>[2x]MIKVEIKPSQAQFTTRSGVSR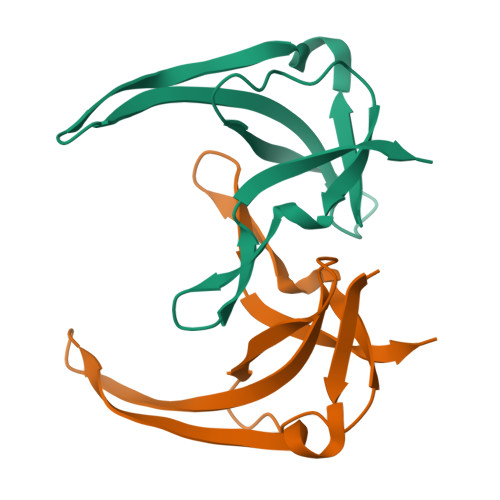QGKPYSLNEQLCYVDLGNEHPVLVKITLDEGQPAYAPGLYTVHLSSFKVGQFGSLMIDRLRLVPAK>SEEVMKDLTSGFIKVLEECKKELNLSESIINDLYNYWKEDYSLLNRDVGCAIVCMSKKLELIDTSGKIHHGNAEDLAKKHGADSEVAAKLVAILHECEKTHDAIEDQCMKALEIAKCFRTNIHELNWAPKMDVVITEVLTEVENLYFQGHHHHHHHHHH[2x]

Insect Pheromone Binding Proteins (PBPs) and Odorant Binding Proteins (OBPs) are found at very high concentrations (up to 10 μM) in the sensillum lymph of insect antennae. These proteins form a large multigene family of small soluble proteins (~ 15 kDa) believed to function as carrier molecules to transport hydrophobic compounds across the sensillum lymph to the membrane-bound odorant receptors present in olfactory sensory neurons (OSNs). Binding proteins that transport important sex pheromones are colloquially named pheromone binding proteins (PBPs). Here, we have produced a functional recombinant PBP from the horticultural pest, Epiphyas postvittana (EposPBP3), and experimentally solved its apo-structure through X-ray crystallography to a resolution of 2.60 Å.

Crystals belonged to the P43 space group, with two molecules in the asymmetric unit. The overall fold of EposPBP3 is conserved with other insect PBPs/OBPs, consisting of six α-helices stabilized by three disulphide bridges (Cys19–Cys54, Cys50–Cys108, and Cys97–Cys117). In contrast to other PBP/OBP structures available in the PDB, both the N-terminus (residues 1–11) and the C-terminus (residues 129–159, which includes the TEV cleavage site and the C-terminal His-Tag) of EposPBP3 appear to be disordered and therefore were not modelled. This may be a consequence of the packing arrangement of the two molecules in the asymmetric unit that brings the N- and C-termini of both molecules in close proximity, where folded N- or C-terminal parts of each monomer would result in steric clashes that are incompatible with the dimer interface observed in the crystals. Towards the end of the refinement, two residual elongated stretches of electron density that could not be interpreted as protein atoms remained at the dimer interface (between the N- and C-termini of both molecules). These were modelled as PEG fragments originating from the crystallisation solution. The structure obtained for EposPBP3 is therefore best described as an intermediate form between form A (N-terminal extended, and C-terminal helix folded) and form B (N-terminal helix folded, C-terminal extended). However, the top part of the cavity (which surrounds and extends above the functional group of the pheromone) appears significantly wider in EposPBP3 than in BmorPBP1. This results from the combination of four amino acid substitutions between the two proteins (Val53Met, Ile62Leu, Lys110Trp and Ala111Thr), and from a slight variation in the position of the exposed loop located between helix 3 and helix 4.>SHDGNSQQGSGSDGGSSMCLELALEGERLCKAGDCRAGVAFFQAAIQAGTEDLRTLSAIYSQLGNAYFYLGDYNKAMQYHKHDLTLAKSMNDRLGEAKSSGNLGNTLKVMGRFDEAAICCERHLTLARQLGDRLSEGRALYNLGNVYHAKGKHLGQRNPGKFGDDVKEALTRAVEFYQENLKLMRDLGDRGAQGRACGNLGNTYYLLGDFQAAIEHHQERLRIAREFGDRAAERRANSNLGNSHIFLGQFEDAAEHYKRTLALAVELGEREVEAQSCYSLGNTYTLLHEFNTAIEYHNRHLAIAQELGDRIGEARACWSLGNAHSAIGGHERALKYAEQHLQLAKELHDPVGESTARVNISDLRKLLGMPDSEPSPTEEEAR[8x];>[8x]SLRFTASTSTPKSGSKIAKRGKKHPEPVASWMSEQRWAGEPEVMCTLQHKSIAQEAYKNYTITTSAVCKLVRQLQQQALSLQVHFERSERVLSGLQASSLPEALAGATQLLSHLDDFTATLERRGVFFNDAKIERRRYEQHLEQIRTVSKDTRYSLERQHYINLESLLDDVQLLKRHTLITLRLIFERLVRVLVISIEQSQCDLLLRANINMVATLMNIDYDGFRSLSDAFVQNEAVRTLLVVVLDHKQSSVRALALRALATLCCAPQAINQLGSCGGIEIVRDILQVESAGERGAIERREAVSLLAQITAAWHGSEHRVP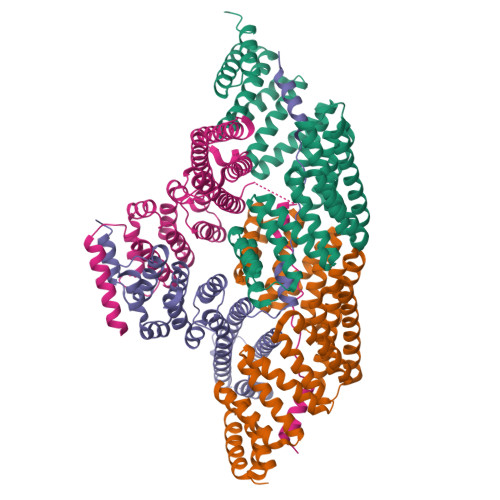GLRDCAESLVAGLAALLQPE>[2x]GSMGKPFFTRNPSELKGKFIHTKLRKSSRGFGFTVVGGDEPDEFLQIKSLVLDGPAALDGKMETGDVIVSVNDTCVLGHTHAQVVKIFQSIPIGASVD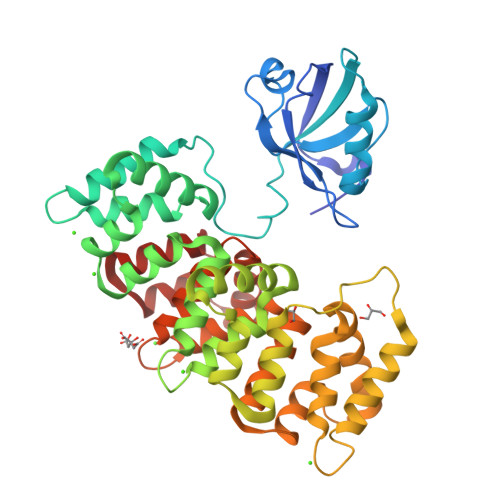LELCRGYPLGSSAYGSVKAYTNFDAERDALNIETAIKTKGVDEVTIVNILTNRSNEQRQDIAFAYQRRTKKELASALKSALSGHLETVILGLLKTPAQYDASELKASMKGLGTDEDSLIEIICSRTNQELQEINRVYKEMYKTDLEKDIISDTSGDFRKLMVALAKGRRAEDGSVIDYELIDQDARDLYDAGVKRKGTDVPKWISIMTERSVPHLQKVFDRYKSYSPYDMLESIRKEVKGDLENAFLNLVQCIQNKPLYFADRLYDSMKGKGTRDKVLIRIMVSRSEVDMLKIRSEFKRKYGKSLYYYIQQDTKGDYQKALLYLCGGDD;> RRVRKLPETTL ETHENO-NADP | C17 H24 N5 O17 P3 | 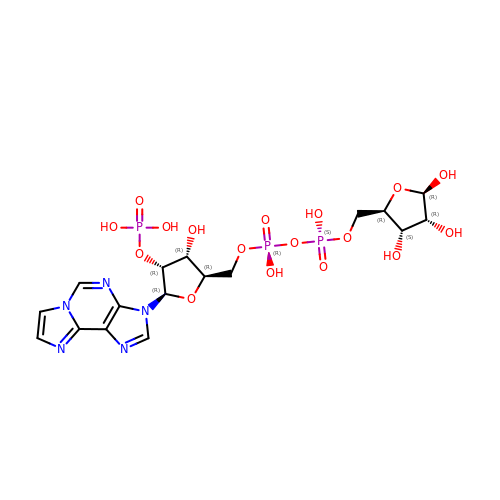KWEQFQACRLGUSH-QJWJOKBXSA-N> HMGRSQNSEFETASDEPIAVIGLSCRLPKASGPQELWQLLDDGASAVTRVPADRETPPSTEEESADGEAAGARWGGFLDRVDTFDAGFFGISPREAAAMDPQQRLVLELSWEALEGAGLVPATLRDTGLGVFVGAARDDYATLYRRREGRAVDHHAMTGLHRSLIANRISYALGAHGPSMVVDTGCSSSLVAVHLACESLRRGESDIALAGGVNLNIAAESARETAAFGGLSPDGQCFTFDARANGFVRGEGGGLVVLKTLRRALADGDLVHGVILASAVNNDGPSDTLTTPSRRAQESLLTRVYRRAGVTPTEVGYVE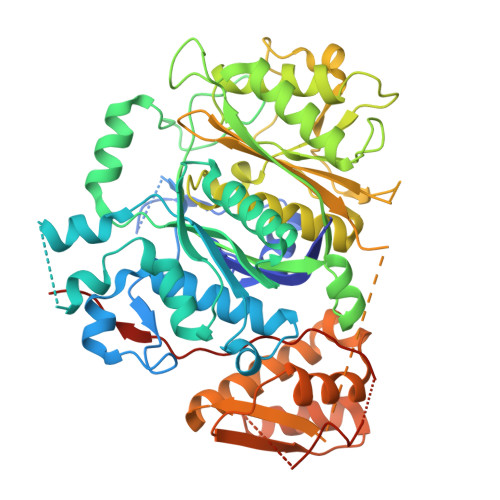LHGTGTKVGDPIEAAALGAVLGTGRDTPLPVGSIKTNIGHLEGAAGIAGLIKALLQLRRRRLVPSLNFSTPNPDIPLDALNLRVQQESAPWATPSGGGRTLVAGVSSFGMGGTNCHVVVSAAPVPEDGETTSEAGATGPDSGPALLPWVVSARSPQALRDQAGRLAAWADSPAGREASPVDIGWSLATSRTHFEYRAVVSGSDRDELVASLRALASGSPVTAAGAVDGRAEPVALLSAVGELFADGYPVDWTAYFAGWPAARVELPTYAFQRSRHWLENVPELAVS> APAVADKADNAFMMICTALVLFMTIPGIALFYGGLIRGKNVLSMLTQVTVTFAL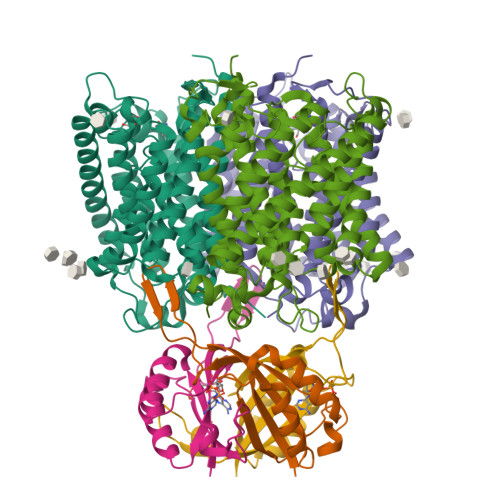VCILWVVYGYSLAFGEGNNFFGNINWLMLKNIELTAVMGSIYQYIHVAFQGSFACITVGLIVGALAERIRFSAVLIFVVVWLTLSYIPIAHMVWGGGLLASHGALDFAGGTVVHINAAIAGLVGAYLIGKRVGFGKEAFKPHNLPMVFTGTAILYIGWFGFNAGSAGTANEIAALAFVNTVVATAAAILGWIFGEWALRGKPSLLGACSGAIAGLVGVTPACGYIGVGGALIIGVVAGLAGLWGVTMLKRLLRVDDPCDVFGVHGVCGIVGCIMTGIFAASSLGGVGFAEGVTMGHQLLVQLESIAITIVWSGVVAFIGYKLADLTVGLRVPEEQEREGLDVNSHGENAYNAGTLVPR;> GPGSMKLVTVIIKPFKLEDVREALSSIGIQGLTVTEVKGFGRQKGHAELYRGAEFSVNFLPKVKIDVAIADDQLDEVIDIVSKAAYTGKIGDGKIFVAELQRVIRIRTGEADEAAL>[2x]GPLGSMIVFVRFNSSYGFPVEVDSDTSIFQLKEVVAKRQGVPADQLRVIFAGKELQNHLTVQNCDLEQQSIVHIVQRPQRKSHETNASGGSEAARGPAAKPTYHSFFVYCKGPCHKVQPGKLRVQCGTCRQATLTLAQGPSCWDDVLIPNRMSGECQSPDCPGTRAEFFFKCGAHPTSDKDTSVALNLITNNSRS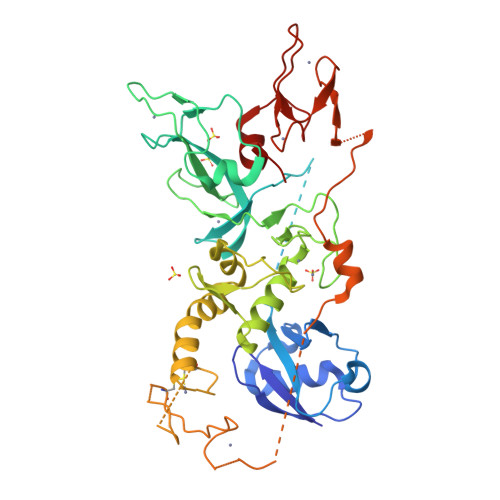IPCIACTDVRNPVLVFQCNHRHVICLDCFHLYCVTRLNDRQFVHDAQLGYSLPCVAGCPNSLIKELHHFRILGEEQYNRYQQYGAEECVLQMGGVLCPRPGCGAGLLPEQGQRKVTCEGGNGLGCGFVFCRDCKEAYHEGECDSMFEASGATSQAYRVDQRAAEQARWEEASKETIKKTTKPCPRCNVPIEKNGGCMHMKCPQPQCKLEWCWNCGCEWNRACMGDHWFDV> RYNDYKLDFRRQQMQDFFLAHKDEEWFRSKYHPDEVGKRRQEARGALQNRLRVFLSLMETGWFDNLLLDIDKADAIVKMLDAAVIKMEGGTENDLRILEQ;> GLECKPRPLHKTCSLFMRNIAPNISRAEIISLCKRYPGFMRVALSEPQPERRFFRRGWVTFDRSVNIKEICWNLQNIRLRECELSPGVNRDLTRRVRNINGITQHKQIVRNDIKLAAKLIHTLDDRTQLWASEPGTPPLPTSLPSQNPILKNITDYLIEEVSAEEEELLGSSGGAPPEEPPKEGNPAEINVERDEKLIKVLDKLLLYLRIVHSLDYYNTCEYPNEDEMPNRCGIIHVRGPMPPNRISHGEVLEWQKTFEEKLTPLLSVRESLSEEEAQKMGRKDPEQEVEKFVTSNTQELGKDKWLCPLSGKKFKGPEFVRKHIFNKHAEKIEEVKKEVAFFNNFLTDAKRPALPE

ARS2 is a direct interaction partner of CBC and together they form a platform for the assembly of co-transcriptional complexes that determine the fate of diverse RNA Pol II transcripts. Our structural analysis shows that ARS2 is made up of two regions, residues 147–270 and 408–763 that co-fold into a structured core with an intervening glutamate-rich region of unknown function that is likely unstructured. The human ARS2 core has an unusual structure comprising a largely helical ‘body’ from which project N- and C-terminal ‘legs’. We find that the RRM domain is required to bind RNA, whereas a basic patch in the C-terminal leg of ARS2 mediates the interaction with FLASH.

Based on the incomplete model, the N-terminal helix was truncated at position 171 with the aim of producing better crystals. ARS2171–270+408–763 crystallised in hexagonal space groups P6522 or P65, diffracting to 3.2 and 3.5 Å resolution, respectively. Selenomethionine-labelled protein was used to solve the structure of the P6522 form using the single-isomorphous replacement methods with anomalous scattering. This required merging data from several crystals to obtain a sufficiently strong anomalous signal. A nearly complete model was built, making use of information from maps calculated in each different crystal form. In mammals, loop A (538-ASEPGT543PPLPTSLPS-552) is highly conserved and proline-rich. In most crystal forms, the loop is disordered presumably due to flexibility. In all crystal structures of hARS2 (except that with loop B deleted), only the first part of the loop is observed with 570-AEEEELL forming helix α10 (‘EEEE helix’). Remarkably, all crystal forms containing loop B, irrespective of space-group, exhibit the same intermolecular crystal contact, in which the acidic ‘EEEE helix’ and the preceding short β-strand pack into the positively charged cradle formed by the RRM β-sheet and the C-terminal extension of the RRM. To accommodate the same intermolecular contact in different crystal-packing environments, some angular flexibility of the loop B structure is required.>MGSSHHHHHHSSGLVPRGSNQPQTTSVLIRKYAIGDYSKLLEGATLQLTGDNVNSFQARVFSSNDIGERIELSDGTYTLTELNSPAGYSIAEPITFKVEAGKVYTIIDGKQIENPNKEIVEPYSVEAYNDFEEFSVLTTQNYAKFYYAKNKNGSSQVVYCFNADLKSPPDSEDGGKTMTPDFTTGEVKYTHIAGRDLFKYTVKPRDTDPDTFLKHIKKVIEKGYREKGQAIEYSGLTETQLRAATQLAIYYFTDSAELDKDKLKDYHGFGDMNDSTLAVAKILVEYAQDSNP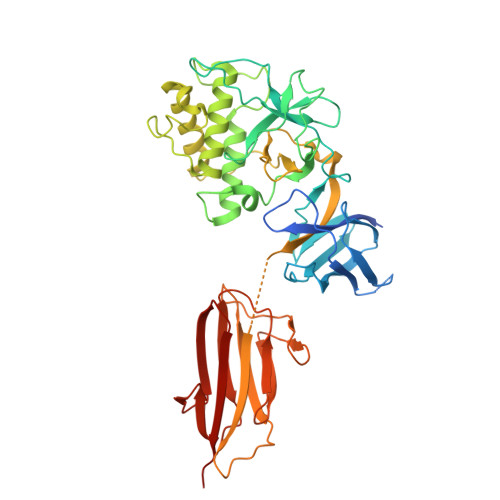PQLTDLDFFIPNNNKYQSLIGTQWHPEDLVDIIRMEDKKEVIPVTHNLTLRKTVTGLAGDRTKDFHFEIELKNNKQELLSQTVKTDKTNLEFKDGKATINLKHGESLTLQGLPEGYSYLVKETDSEGYKVKVNSQEVANATVSKTGITSDETLAFENNKEPVVPT[2x]> MELSEGELSHTSSSSSFVPVDQRQLQDAIQIIDENKHFNTGILDYINKTSPADVGNNYHIISVFGSQSTGKSTLLNRLFNTNFDVMDELNRQQTTKGIWLAYSPVVSTTLGHTTSKSNILVMDVEGTDGRERGEDQDFERKAALFALSTSEVLIINIWETQVGLYQGANMGLLKTVFEVNLSLFGKSKLETHNDHKVLLLIVIRDHVGVTPVESLAKTFTLDLQNMWSSLAKPAELEHLQFADFFDVTFHALNHKVLQPKEFGEGINRLGDRLVVSNELFKPEYHHDVPIDGWTMYAERCWEQIETNKDLDLPTQQILVAQFKCDEIVESVFQEFLTKYQHHFKEVDAAPDFEELGALFADLRQDAFEDYDASASRYNKAVYEQKRKKLRWLINDKLKEVFDVHAKNLCNTLLEKFEKDLVALKGKDFAVNVKTLSTKLVEDVNFQVSLMSLQGDLSLDEIILALTKDIDAIVAKQQVVELNSIVNKSVKKLSASLSKSIQFELGDPNEETWDNVLQQFKGVYEKFGGDFGLGTSSTQNQQAIEKFKFKSWCQFYDVTHKLISREKLLALLQDRFDDKFRYDENGLPKLYLNEQDLEKTFAVAKQHALQVLPILTFAKLADGSEIVPDYDIFDSKLRE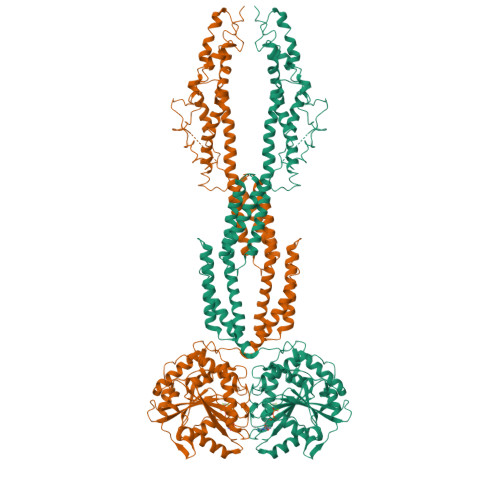QFLGGYDDSDDEEDHCFAEIITEQEKLEVLAKFKKEVDAKYIETKRSIVQHITQ>LKCNKLVPLFYKTCPAGKNLCYKMFMVATPKVPVKRGCIDVCPKSSL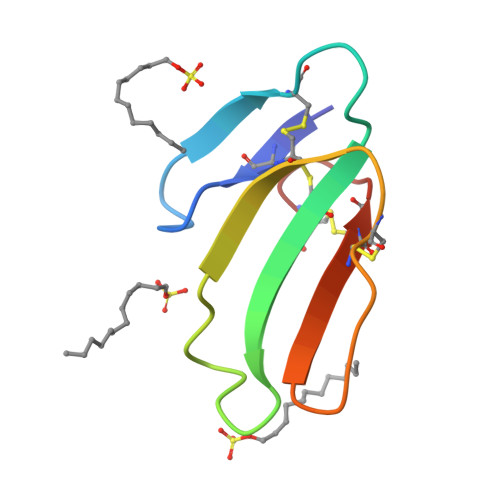LVKYVCCNTDRCN[3x]O-[(2S)-2-amino-3-hydroxypropanoyl]-N-(2,3-dihydroxybenzoyl)-L-serine | C13 H16 N2 O8 | 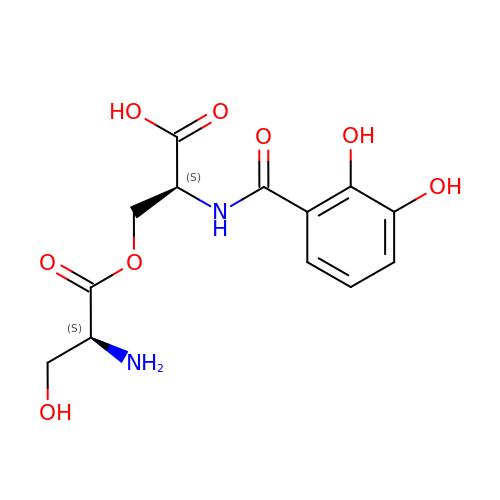NNOZTAPXJBUXBD-YUMQZZPRSA-N> EDMPVERILEAELAVEPKTETYVEANMGLNPSSPNDPVTNICQAADKQLFTLVEWAKRIPHFSELPLDDQVILLRAGWNELLIASFSHRSIAVKDGILLATGLHVHRNSAHSAGVGAIFDRVLTELVSKMRDMQMDKTELGCLRAIVLFNPDSKGLSNPAEVEALREKVYASLEAYCKHKYPEQPGRFAKLLLRLPALRSIGLKCLEHLFFFKLIGDTP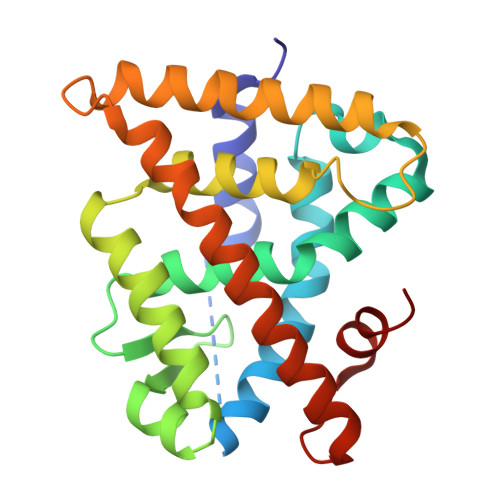IDTFLMEMLEAP>MSLREVALKILIVEDDTDAREWLSTIISNHFPEVWSAGDGEEGERLFGLHAPDVIITDIRMPKLGGLEMLDRIK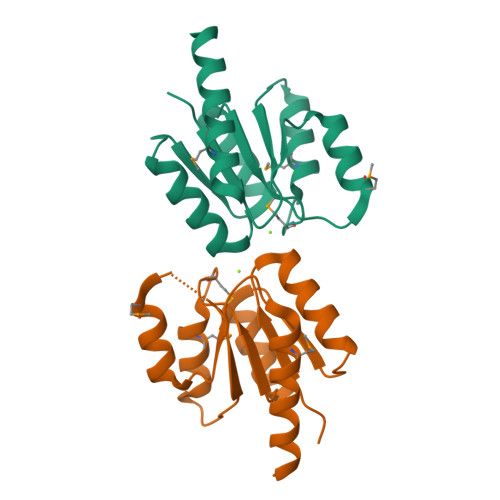AGGAKPYVIVISAFSEMKYFIKAIELGVHLFLPKPIEPGRLMETLEDFRHIKLAKEGHHHHHH[4x]> MRGGALLCGQVQDEIEQLSRESSHFSLSTGILPSLGARSNRRVKLRRFVVSPYDHKYRIWEAFLVVLVVYTAWVSPFEFGFLRKPRPPLSITDNIVNAFFAIDIIMTFFVGYLDKSTYLIVDDRKQIAFKYLRSWFLLDLVSTIPSEAAMRISSQSYGLFNMLRLWRLRRVGALFARLEKDRNFNYFWVRCAKLVCVTLFAVHCAACFYYLIAARNSNPAKTWIGANVANFLEESLWMRYVTSMYWSITTLTTVGYGDLHPVNTKEMIFDIFYMLFNLGLTAYLIGNMTNLVVHGTSRTRNFRDTIQAASNFAHRNHLP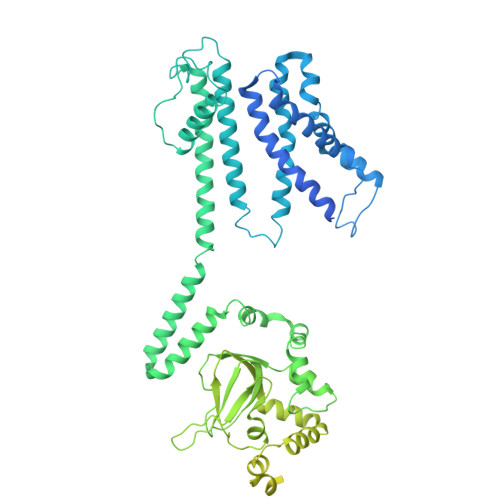PRLQDQMLAHLCLKYRTDSEGLQQQETLDALPKAIRSSISHFLFYSLMDKVYLFRGVSNDLLFQLVSEMKAEYFPPKEDVILQNEAPTDFYILVNGTADLVDVDTGTESIVREVKAGDIIGEIGVLCYRPQLFTVRTKRLCQLLRMNRTTFLNIIQANVGDGTIIMNNLLQHLKEMNDPVMTNVLLEIENMLARGKMDLPLNLCFAAIREDDLLLHQLLKRGLDPNESDNNGRTPLHIAASKGTLNCVLLLLEYHADPNCRDAEGSVPLWEAMVEGHEKVVKVLLEHGSTIDAGDVGHFACTAAEQGNLKLLKEIVLHGGDVTRPRATGTSALHTAVCEENIEMVKYLLEQGADVNKQDMHGWTPRDLAEQQGHEDIKALFREKLHERRVHIETSSSVPILKTGIRFLGRFTSEPNIRPASREVSFRIRETRARRKTNNFDNSLFGILANQSVPKNGLATVDEGRTGNPVRVTISCAEKDDIAGKLVLLPGSFKELLELGSNKFGIVATKVMNKDNNAEIDDVDVIRDGDHLIFATDS AtzH is the first DUF3225 family protein that has been shown to possess a catabolic function, likely decarboxylating the product of AtzEG-mediated deamination of 1-carboxybiuret as part of the cyanuric acid mineralization pathway. The data presented here imply that AtzH is a decarboxylating, 1,3-dicarboxyurea amidohydrolase. AtzH belongs to NTF2-fold superfamily, which contains 38 protein families, including the AtzH family: DUF3225 (DUF: domain of unknown function). Size exclusion chromatography performed on AtzH after removal of the his-tag, suggested that the native protein had a molecular mass of ~ 29 kDa, consistent with a dimer (2 x 14,655 kDa).

As 1,3-dicarboxyurea is unstable, it was not possible to produce crystals of AtzH in its presence. The wild-type and variants were co-crystallized with 1,3-dicarboxyacetone, a stable structural analogue of 1,3-dicarboxyurea. The hydrogen bonding network is largely as predicted for 1,3-dicarboxyurea, and Tyr22 is well positioned as the catalytic residue. The Arg46Ala and Arg46Lys variants both increased the rate of ammonia production by the cascade, but to a lesser degree than that of the wild-type AtzH. This may suggest that Tyr22 is the catalytic amino acid residue in AtzH, possibly acting as a proton donor (consistent with the catalytic role of tyrosine in other enzymes), with Arg46 fulfilling a non-critical function As the substrate analog binds between Arg46 and Tyr22, it seems unlikely that Arg46 has a role in activating Tyr22 (noting that the substrate analog may not adopt exactly the same conformation as the bound substrate). However, this positioning of the active site residues relative to the bound analog is similar to that of the catalytic residues in inverting β-glycosidases that use an acid-base catalytic mechanism, and it is plausible that that a similar mechanism may be used here. As yet its catalytic mechanism is not known, but our results suggest it involves the action of Tyr22 and Arg46, and that these amino acid residues are positioned relative to the substrate in a manner consistent with an acid-base mechanism.

>MGSSHHHHHHHSSGLVPRGSHHMLEMQINLPEVHAEVTAQFVRYEKALTSNDTAVLNELFWNSPQTLRYGATENLYGYEAIAGFRATRSPNNLEKEIVRTVITTYGHDFATANIEFRRLSHSQLTGRQSQTWMRTSQGWRVVAAHVSLIALPVS[12x]> MGRVYYGGVERTYLYRGRILNLALEGRYEIVEHKPAVAVIAL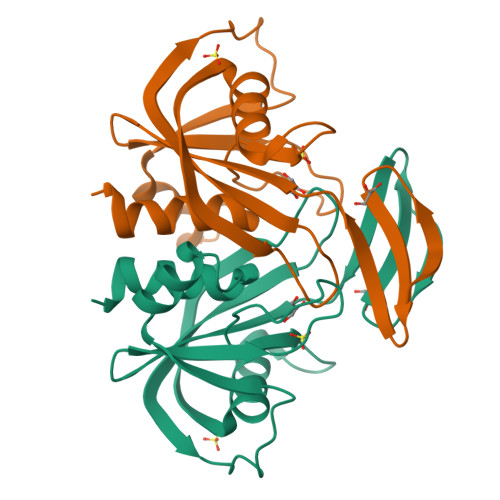REGRMLFVRQMRPAVGLAPLEIPAGLIEPGEDPLEAARRELAEETGLSGDLTYLFSYFVSPGFTDEKTHVFLAENLKEVEAHPDEDEAIEVVWMRPEEALERHQRGEVEFSATGLVGVLYYHAFLRGR3,6,9,12,15,18,21,24,27-nonaoxaheptatriacontan-1-ol | C28 H58 O10 | 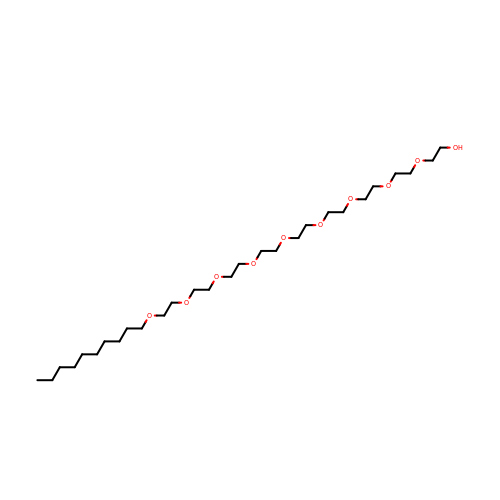MEPDRUVBZDYVEU-UHFFFAOYSA-N> ITLLTLIKTAEHWARQDIRTIEDSKLRALL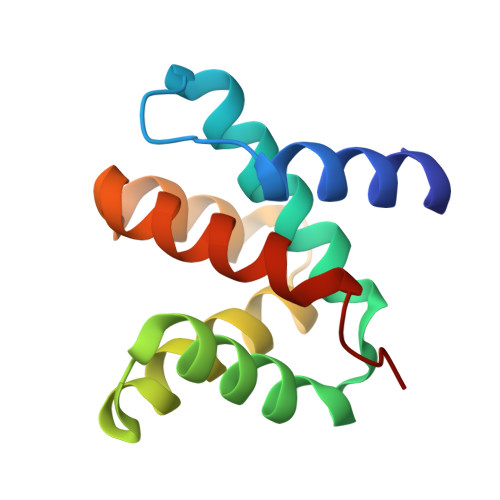TLCAVMTRKFSKSQLSLLCETHLRREGLGQDQAEPVLEVYQRLHSDKGGSFEAALWQQWDRQSLIMFITAFLNIALQLPCES> MKDFSKDFLFGVATASYQVEGAYNEDGRTMSIWDTFSRQDGKVYKSHNGDVACDHYHLYKDDVKMMKDLGIEAYRFSIAWPRIFPAKGQYNPKGMDFYKRLTDELLKNDIKPFATIYHWDLPQWADDLGGWLNREIVEWYGEYAEKLFSELGGYIKNWITLNEPWCSSFLSYFIGEHAPGHKDLGEALLVSHNLLLSHGKAVEIFRGLNLDDSKIGITLNLNEVFPASDSDDDKVAAQIADGFQNRWFLDPLFKGKYPQDMVEYFGKYAKVDFINDEDLKLISQKLDFLGVNYYTRAVVQKGNDGLLDAVQIDPGNERTEMGWEIYPESLYNILMRLKREYTYDMPLYITENGAAFNDVVEDDGRVHDEKRVEFLKQHFKEAKRFLNDGGNLKGYFVWSLMDNFEWAHGYSKRFGIVYVDYETEKRILKDSALWYKDLISTRTI

β-glucosidases (Bgls, β-d-glucopyranoside glucohydrolases, E.C. 3.2.1.21) cleave β-1,4-glycosidic bonds in disaccharides or glucose-substituted polysaccharides, thereby releasing non-reducing terminal glucosyl residues. Bgl proteins have a TIM-barrel fold. The substrate-binding pocket can be divided into the glycone, aglycone, and gatekeeper regions; in addition, the bound sugar substrate is cleaved via a retention mechanism using two glutamate residues. Four loops are present above the Bgl substrate-binding pocket, forming a large cavity for the nascent substrate to access.

Two different space groups of TsaBgl crystals containing triclinic P1 and orthorhombic P212121 were obtained at pH 7.5 and 8.0, respectively. Two TsaBgl-P212121 structures were processed up to 1.5 and 1.6 Å, with Rwork/Rfree of 0.1546/0.1712 and 0.1506/0.1762, respectively. Particularly, the L3 loop exhibited two structurally distinct conformations, one where it was oriented towards the substrate-binding pocket (folded L3 loop) and the other where it was oriented towards the solvent direction, i.e., away from the substrate-binding site (straight L3 loop). In the P1 and P212121 crystals, the L3 loop regions of the TsaBgl-Data I (folded L3 loop conformation) and TsaBgl-Data III (straight L3 loop conformation) chain A molecules, which showed the most significant differences in L3 loop conformation, were carefully analyzed. While the straight L3 loop had a relatively straight loop structure in the direction pointing away from the substrate-binding pocket, the folded L3 loop was oriented toward the substrate-binding pocket. Conversely, the substrate accessible width of the substrate-binding pocket entrance with the straight L3 loop conformation was approximately 35 Å, and the proximate distance between the L2 and L3 loops was approximately 7 Å. We speculated that the straight L3 loop conformation made the substrate entrance wider, thereby providing easier access to the substrate than the folded conformation. In contrast, in the straight L3 loop, both the Leu306 and Leu307 residues maintained hydrophobic interactions with surrounding hydrophobic residues. A Tris molecule was shown to act as an inhibitor of TsaBgl β-glucosidase activity. This molecule was found to bind to all the active sites in the TsaBgl glycone region.2-(6-morpholin-4-ylpyrimidin-4-yl)-4-(1,2,3-triazol-1-yl)pyrazol-3-ol 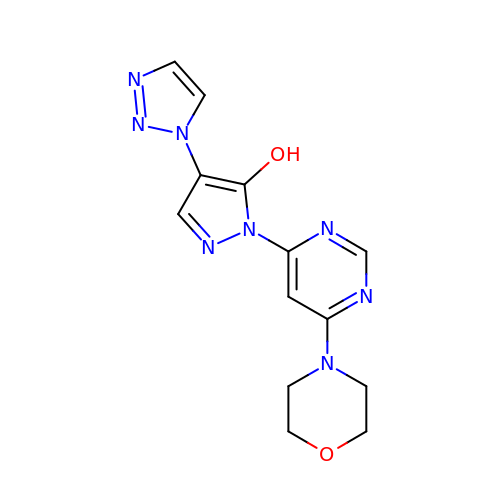| C13 H14 N8 O2 | NTIRTFLRBFAPSX-UHFFFAOYSA-N(2~{S})-2-[3-(4-chlorophenyl)sulfanylpropanoylamino]-3-methyl-butanoic acid | C14 H18 Cl N O3 S | 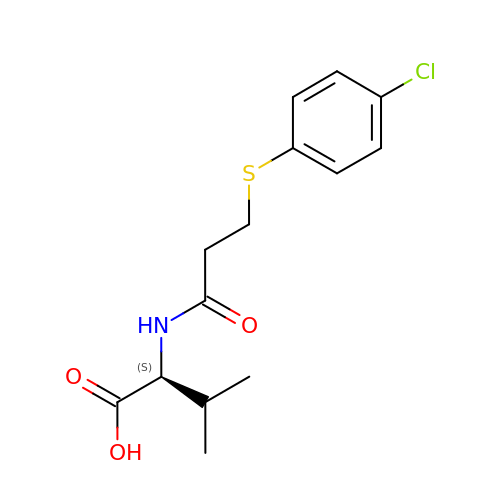ZRYCUODJUIAJCI-ZDUSSCGKSA-N1-(4-cyanophenyl)-3-[[3-(2-cyclopropylethynyl)imidazo[2,1-b][1,3]thiazol-5-yl]methyl]urea 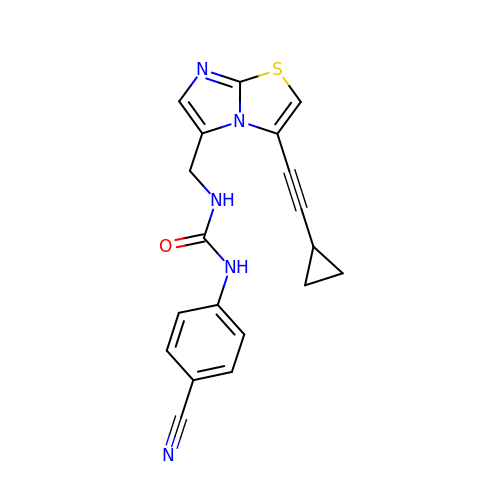| C19 H15 N5 O S | JCNMORLJVKCDDB-UHFFFAOYSA-N> METFDPTELPELLKLYYRRLFPYSQYYRWLNYGGVIKNYFQHREFSFTLKDDIYIRYQSFNNQSDLEKEMQKMNPYKIDIGAVYSHRPNQHNTVKLGAFQAQEKELVFDIDMTDYDDVRRCCSSADICPKCWTLMTMAIRIIDRALKEDFGFKHRLWVYSGRRGVHCWVCDESVRKLSSAVRSGIVEYLSLVKGGQDVKKKVHLSEKIHPFIRKSINIIKKYFEEYALVNQD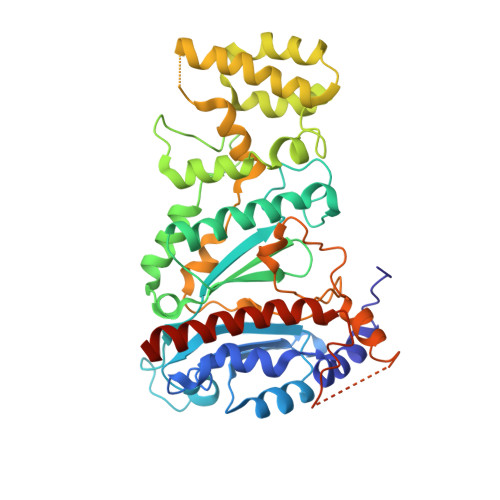ILENKESWDKILALVPETIHDELQQSFQKSHNSLQRWEHLKKVASRYQNNIKNDKYGPWLEWEIMLQYCFPRLDINVSKGINHLLKSPFSVHPKTGRISVPIDLQKVDQFDPFTVPTISFICRELDAISTNEEEKEENEAESDVKHRTRDYKKTSLAPYVKVFEHFLENLDKSRKGELLKKSDLQKDF> QGPSSPMDSSRRQYQEKYKQVEQYMSFHKLPADFRQKIHDYYEHRYQGKMFDEDSILGELNGPLREEIVNFNCRKLVASMPLFANADPNFVTAMLTKLKFEVFQPGDYIIREGTIGKKMYFIQHGVVSVLTKGNKEMKLSDGSYFGEICLLTRGRRTASVRADT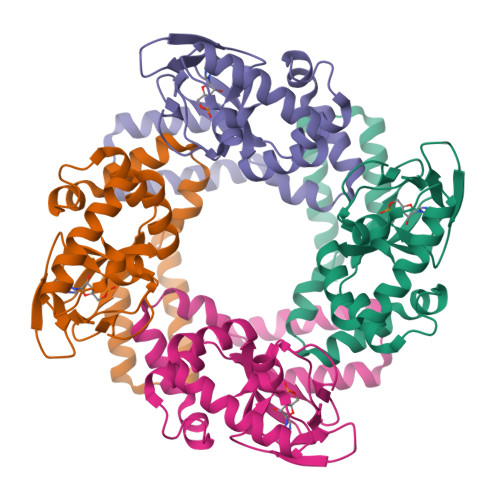YCRLYSLSVDNFNEVLEEYPMMRRAFETVAIDRLDRIGKKNSILLH Proteins containing a FIC domain catalyze AMPylation and other post-translational modifications (PTMs). Among these, Bartonella effector proteins (Beps) comprise a particularly diverse ensemble of FIC domains that subvert various host cellular functions. The FIC fold comprises eight conserved α-helices and encompasses a characteristic active site loop between helices α4 and α5 that forms most of the catalytic center and the substrate binding pocket. Additionally, FIC domains generally contain a β-hairpin between helix α2 and helix α3 that is referred to as the “flap” and mediates docking of a target segment in extended conformation via β-strand augmentation.

The structures of Bhe_BepA, Bcl_Bep1, Bqu_BepC, and Btr_BepC exhibit all features defining a FIC AMP transferase as described in the first chapter and elsewhere. Indeed, the complex of Btr_BepC with AMPPNP demonstrates competent tri-phosphate nucleotide binding as has been observed for, e.g., the inhibition-relieved VbhT/VbhA(E24G) complex. However, BepC proteins are special in that they have a lysine instead of a Mg2+-coordinating aspartate/glutamate in the FIC motif. The structure shows that this lysine (K150) is interacting directly with the α-phosphate. Thus, BepC proteins appear to require no divalent cation for substrate binding, in contrast to all FIC AMP transferases characterized so far. The structure also verifies that a cysteine (C185) can substitute the ribose binding serine (last position of the active site motif used in Figure 6B). For BepC, despite its canonical signature motif, no catalytic activity has yet been found, but its BepFIC domain mediates protein–protein interaction with the RhoGEF GEF-H1, thereby activating RhoA signaling. Btr_BepC FIC with AMPPNP crystals were grown from a solution of 10% w/v PEG 8000, 20% v/v ethylene glycol, 0.1 M MES/imdazole, pH 6.5, and 0.02 M each of sodium L-glutamate, DL-alanine, glycine, DL-lysine, and DL-serine. Data for Btr_BepC FIC with AMPPNP were collected on a Rigaku Saturn 944 + detector at a wavelength of 1.5418 Å with our in-house source (Rigaku FR-E + Superbright rotating anode).

> MAHHHHHHMEQNYLYKGTTTLKNKYGIKDPNKLYERCNHDVVKEAVNFRHEPPPQNFDAAYLSLIHWSLFHKTFEWAGHTRDTSFTFEDGTTARMPAMRPKGYEAPFAIGPQIKKELKQLEKTLNQKNNLKGLSHQEFAENAADVFMALEHAHPFRKGNGRANRMFMEKLGQAAGHTVDFSFITKGRMTTACIEAMQYGNSQPMKDLFEDITHPQKSVILKEFISQM> MRNEMHLQFSARSENESFARVTVAAFVAQLDPTMDELTEIKTVVS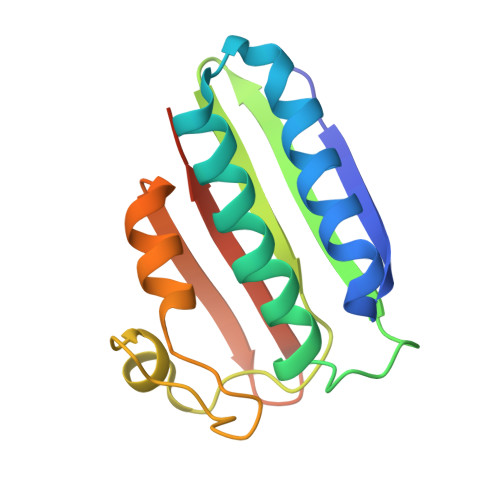EAVTNAIIHGYNNDPNGIVSISVIIEDGVVHLTVRDEGVGIPDIEEARQPLFTTKPELERSGMGFTIMENFMDEVIVESEVNKGTTVYLKKHGIHHHHHH> PESELIRQSWRVVSRSPLEHGTVLFARLFALEPSLLPLFQYNGRQFSSPEDSLSSP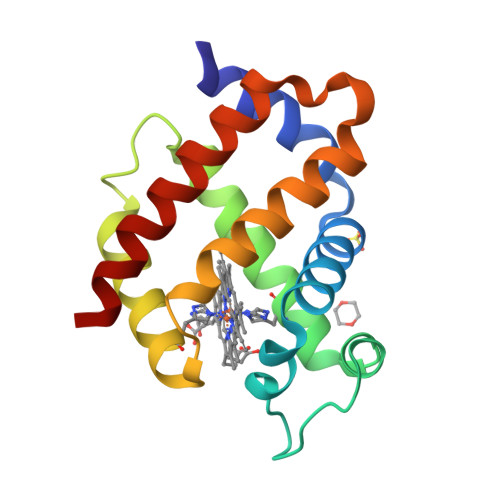EFLDHIRKVMLVIDAAVTNVEDLSSLEEYLTSLGRKHRAVGVRLSSASTVGESLLYMLEKSLGPDFTPATRTAWSRLYGAVVQAMSRGWD> MISARAVHRFLRNPNLETGAAFRAGTRFDPFKNTLTVLKDPQNGRTLYLIGTTNSSTLLANRTKDLVQKEKPDAVFVQTNKEWWNLAKNIQDVKCQQELNRYNDLLSQAYTLSLDNTIRNLVFKAKFYSWLFVINWFKAFPDDFHPFIPGLEMKFAIEEANKQNIPVVLGGLEVDDVTLSALKVEPRLDPFSQLYYGYRALHNSFWRRE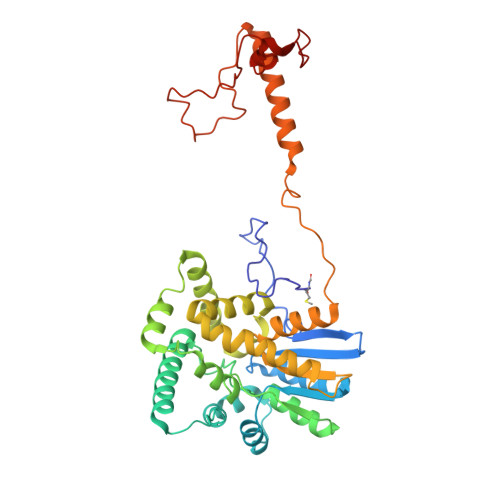HFDNYATLDVVGGEAYAESMDRFRTNWFVKYFEKLAPYQKKIIVDQKDLDLFYALYRDTPGKKIVAVVNQWHVPGIENHWKSATNTHEPLKAINPIGDMDINKYMESQLVNDTLRAFVSKVGKTEPATWKNYSTIYHKDNYEAERVRHVAFVDHKDPHMYHGLPQDYDDNIKPKHH>[4x]MSTGPDFIYDDRPAAVSSTFNPEKGYMDFITAYGKNINADNVRIFFLNHKKAKDSLKGSPKVEVDLQFGTL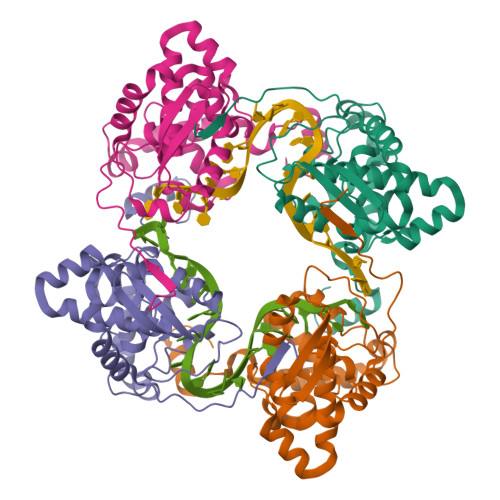RVKVVNNHNPRNRDNPVADNAITLHRLSGYLAKWCFDEIDHGQIEEAEVKSKVVIPLAEAKGCKWGDGVALYLAFAPGAEMFLKDFEFYPLAIDIQRVVKDGMDITFMRKVLKQRYGTKTADDWMISEVTAIQSAVKVVAKLPWAKAGFTAAAKNFLAKFNISV Except for an N-terminal region, Prp3 is highly conserved from yeast to human and contains a C-terminal domain of unknown function (DUF1115; PFAM ID PF06544). Here, we showed that Prp3 orthologs contain a C-terminal U4/U6 di-snRNA binding region that encompasses a DUF1115 domain and a preceding peptide rich in basic residues. Our crystal structure and targeted mutational analyses demonstrate that the DUF1115 domain acts as a ssRNA-binding domain that specifically recognizes the first 10 nts of the U6 3′-overhang. Our results indicate how Prp3 functionally bridges U4/U6 and U5 in the tri-snRNP by Prp3-RNA interactions on one side and Prp3-protein interactions on the other.

To elucidate the molecular mechanism underlying U4/U6 di-snRNA binding by yPrp3CTF, we determined its crystal structure in complex with yU4/U6stem II+10nt at 3.25 Å resolution. Residues 335–468 of yPrp3CTF and all nts (G81-U90) of the yU6 3′-overhang were well ordered in the two complexes contained in an asymmetric unit. In both complexes, the single-stranded (ss) yU6 3′-overhang arches across helix α1 and strand β5 of yPrp3CTF, running below the long β3a/β3b hairpin. Its binding surface on the protein is carpeted by an electropositive surface potential. The yU6 3′-overhang can be divided into three sections, between which its backbone changes directions on the surface of yPrp3CTF. Nts G81-A83 (section 1) stack on the terminal U80U6-A1U4 base pair of stem II and run diagonally from the N-terminus of helix α2 to the N-terminus of helix α1; nts C84-G86 (section 2) are positioned perpendicular across the N-terminal end of helix α1; nts U87-U90 (section 3) run along the exposed edge of strand β5 and the C-terminus of helix α1. As a consequence, the end of the U6 3′-overhang is directed via two ca. 90 ° kinks back towards stem II. Notably, the unusual doubly-kinked RNA conformation is stabilized by protein elements that expand the core ferredoxin fold in yPrp3, that is, the β3a/β3b hairpin, strand β5 and helix α3 (details below). The guanidinium group of R353 (helix α1) engages in hydrogen bonds to the Watson-Crick face of C85 (atoms O2 and N3) and to the Hoogsteen face of G86 (atoms O6 and N7). Upon RNA binding, the β3a/β3b hairpin moves closer to the yPrp3CTF core domain to engage in direct interactions with the RNA and the H409 side chain in this element turns on top of the C84 base.

>[2x]GAMVVKDQVDLRKRKHLEENERRHEDAIKRRKEAVNMNVEKPTVYHCKVFQFKNLQNPKIRFKLKMNSKELSLKGLCLRIRDDGPGIIIVVGNEKSCKFYENLVMKRIKWNEDFELHTNTGDIKMDMHNNSISKTWEGYLQDCKFKGWFMKVCNDQDSLLRTLGQFDSEHFYSPVQT>AEAGITGTWYNQLGSTFIVTAGADGALTGTYESAVGNAESRFVLTGRYDSAPATDGSGTALGWTVAWKNNYRNAHSATTWSGQYVGGAEARI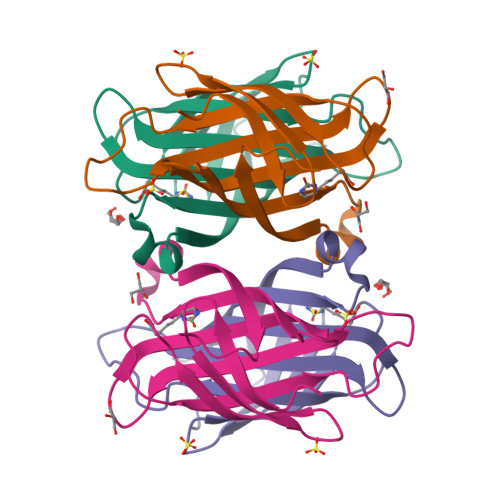NTQWLLTSGTTEANAWKSTLVGHDTFTKVKPSAAS[2x]> MISDIRKDAEVRMDKCVEAFKTQISKIRTGRASPSLLDGIVVEYYGTPTPLRQLASVTVEDSRTLKINVFDRSMSPAVEK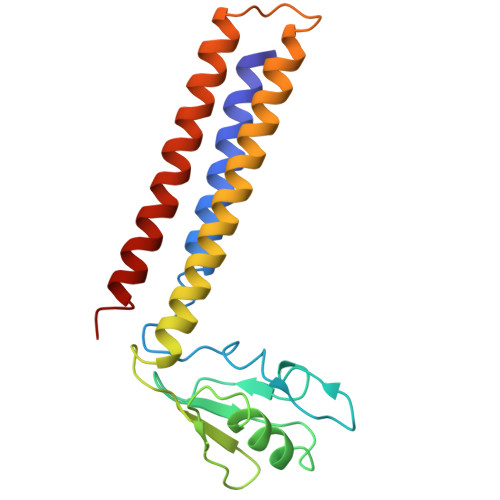AIMASDLGLNPNSAGSDIRVPLPPLTEERRKDLTKIVRGEAEQARVAVRNVRRDANDKVKALLKDKEISEDDDRRSQDDVQKLTDAAIKKIEAALADKEAELMQF>GAMGKSEGVTIEFKIVGLNKKLKVFTTCPHTLFGASFCA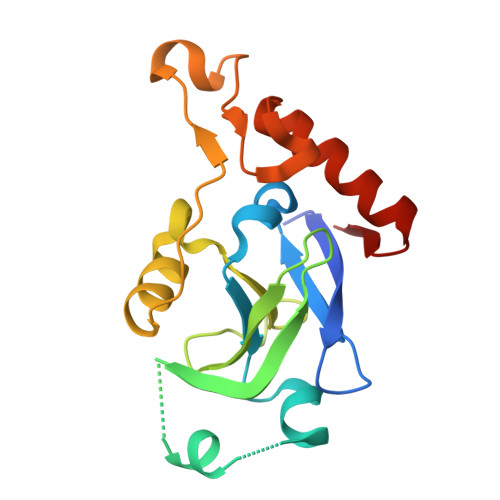VAIEHPIVQDLMSKEIQDLISSIKIQGKNNEKVGIYTGLNVKHPFLDKELPLYVANFVLMEYREGAIFGCPAHDQRDFEFAQEYDLPIIPVISSARLGIEEYTNNSIMFNSEFLNGLTVSEARKVIVEKLEEKGIGKKTI[4x]> MH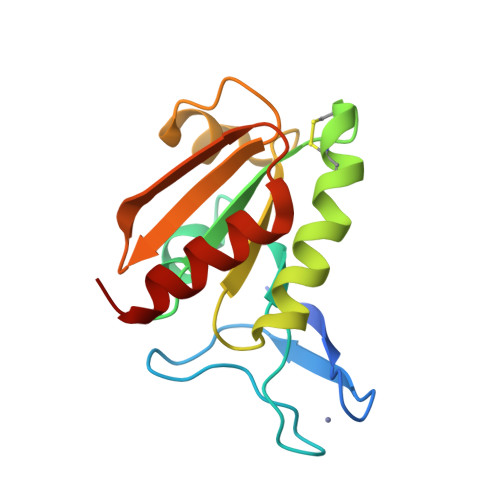HHHHHSDILTCTHCQAKNRVGAVPAGQVPSCARCGAALPWLHDGTDATFEQDLQTSVPVLVDFWAPWCGPCRVMGPVLEDLARDLPGKVRVVKVNVDENPRTAARFEVRSIPTLLMFKDGEEVDQMVGVTQKAALRARVEHLNQLS The HIV-1 Trans-Activation Response element (TAR) RNA, located at both ends of its RNA genome, is one of the most conserved RNA structural elements in retroviruses. It assumes multiple, dynamic conformations to carry out critical functions in several stages of the HIV-1 life cycle, including reverse transcription, proviral transcription, genome dimerization and packaging, viral translation, and immune suppression, etc. Here, we report crystal structures of the full-length HIV-1 TAR which reveal substantial conformational mobility in its three conserved bulges and in its lower stem, which coordinately maintain the structural fluidity of the entire RNA. We find that TAR RNA is a robust inhibitor of PKR, and primarily uses its lower stem to capture and sequester PKR monomers, preventing their dimerization and activation.

Herein we report four crystal structures of this 57-nt RNA, both free and bound to HIV-1 Tat. In both cases, Tat induces a substantial conformational change which positions U23 in the major groove of the A27-U38 pair, forming a base triple. In both the co-crystal and NMR structures, the central U23•A27-U38 base triple is sandwiched and stabilized by two G-C pairs (G26-C39 and G28-C37), as well as by two Tat arginine side chains (R52 and R56/R49) that are co-planar with the flanking G-C pairs. The guanidinium groups of R52 and R56/R49 not only form hydrogen bonds with the Hoogsteen edges of G26 and G28 but also stack with the base triple via cation-π and van der Waals interactions. Essentially, these two flat guanidiniums mimic third nucleobases in the major groove (like U23), forming two pseudo-base triples (R52•G26-C39 and R56/R49•G28-C37) which sandwich the central bona fide U23•A27-U38 base triple (triangles). Unlike the NMR structure, the crystal structure places R49 of Tat in direct contact with G21, making yet another arginine fork interaction with the Hoogsteen edges similar to R52 and R56. Tat projects the guanidinium groups of three arginines, R49, R52, and R56, to recognize the Hoogsteen edges of three guanines, G21, G26, and G28, respectively, with R52 making a central, indispensable contact. Strikingly, while the flanking R49A and R56A substitutions each had only ~ 3-fold effects on binding, the central R52A reduced binding by more than 400 fold, in agreement with its in vivo importance for Tat-mediated HIV trans-activation. Any nucleobase at position 24 sufficiently supports Tat binding, consistent with its solvent exposure and cation-π stacking with R55 of Tat in the co-crystal structure. Although our Tat helix-TAR structure seems to require the crystal lattice for stabilization, it demonstrates the structural feasibility for a conformationally constrained Tat helix to fit in the TAR major groove, induce the U23 triple formation, and make highly similar contacts.

> GISYGRKKRRQRRRAHQ>[2x]SNSLHWPTSLPSGDAFSSVGTHRFVQKVEEMVQNHMTYSLQDVGG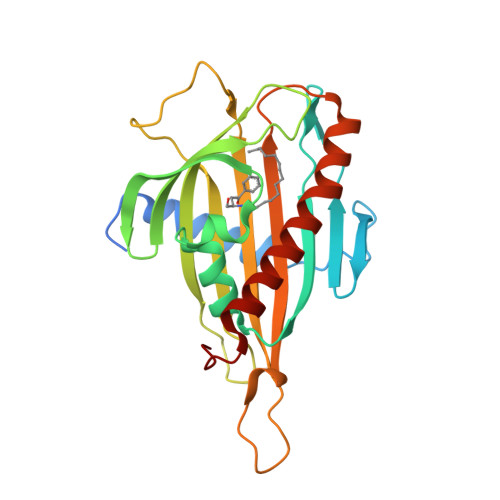DANWQLVVEEGEMKVYRREVEENGIVLDPLKATHAVKGVTGHEVCNYFWNVDVRNDWETTIENFHVVETLADNAIIIYQTHKRVWPASQRDVLYLSVIRKIPALTENDPETWIVCNFSVDHDSAPLNNRCVRAKINVAMICQTLVSPPEGNQEISRDNILCKITYVANVNPGGWAPASVLRAVAKREYPKFLKRFTSYVQEKTAGKPILF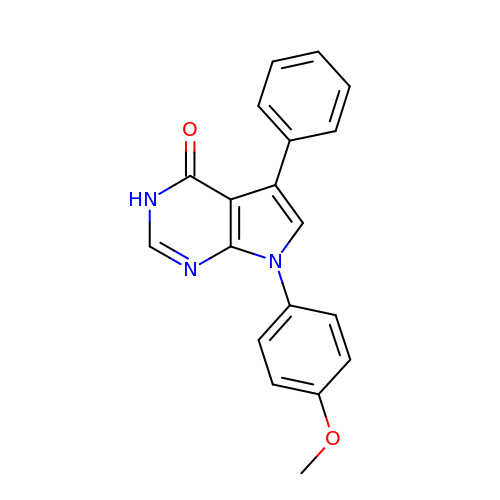7-(4-methoxyphenyl)-5-phenyl-3,7-dihydro-4H-pyrrolo[2,3-d]pyrimidin-4-one | C19 H15 N3 O2 | VAOBJTRTUSWVKW-UHFFFAOYSA-N>[3x]MTPASYNLAVRRAAPAVVNVYNRGLNTNSHNQLEIRTLGSGVIMDQRGYIITNKHVINDADQIIVALQDGRVFEALLVGSDSLTDLAVLKINATGGLPTIPINARRVPHIGDVVLAIGNP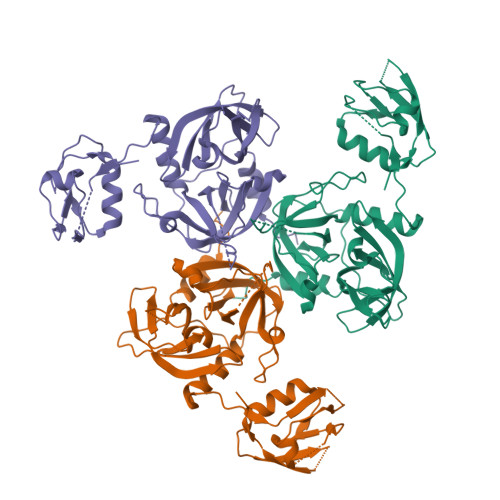YNLGQTITQGIISATGRIGLNPTGRQNFLQTDASINHGNSGGALVNSLGELMGINTLSFDKSNDGETPEGIGFAIPFQLATKIMDKLIRDGRVIRGYIGIGGREIAPLHAQGGGIDQLQGIVVNEVSPDGPAANAGIQVNDLIISVDNKPAISALETMDQVAEIRPGSVIPVVVMRDDKQLTLQVTIQEYPATN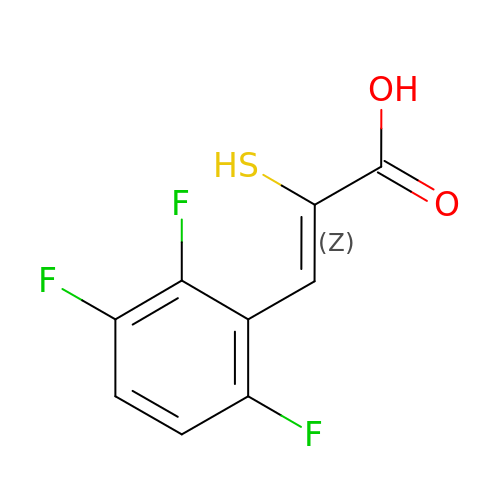(~{Z})-2-sulfanyl-3-[2,3,6-tris(fluoranyl)phenyl]prop-2-enoic acid | C9 H5 F3 O2 S | AFXJYTIRLSCBCG-CLTKARDFSA-N> DFESPNI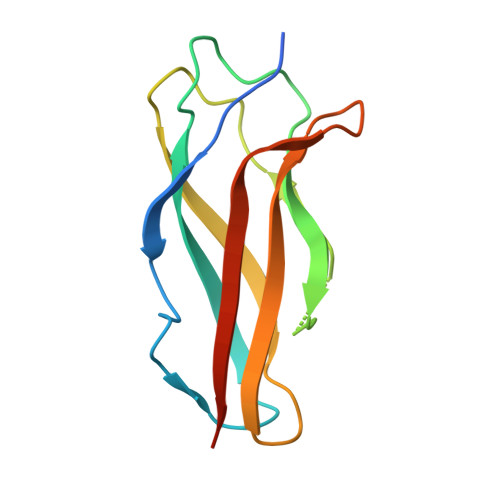SVPSMSFVEDVTIGEGESIPPDTQFVKTWRIQNSGAEAWPPGVCLKYVGGDQFGHVNMVMVRSLEPQEIADVSVQMCSPSRAGMYQGQWRMCTATGLYYGDVIWVILSVEVGGLL> AGNDLLSCLTFNGVRNHTVFSADSDSDFNRFLHLSIQNPLFQNSLISKPSAIILPGSKEELSNTIRCIRKGSWTIRLRSGGASYEGLSYTSDTPFILIDLMNLNRVSIDLESETAWVESGSTLGELYYAITESSSKLGFTAGWCPTVGTGGHISGGGFGMMSRKYGLAADNVVDAILIDANGAILDRQAMGEDVFWAIRGGGGGVWGAIYAWKIKLLPVPEKVTVFRVTKNVAIDEATSLLHKWQFVAEELEEDFTLSVLGGADEKQVWLTMLGFHFGLKTVAKSTFDLLFPELGLVEEDYLEMS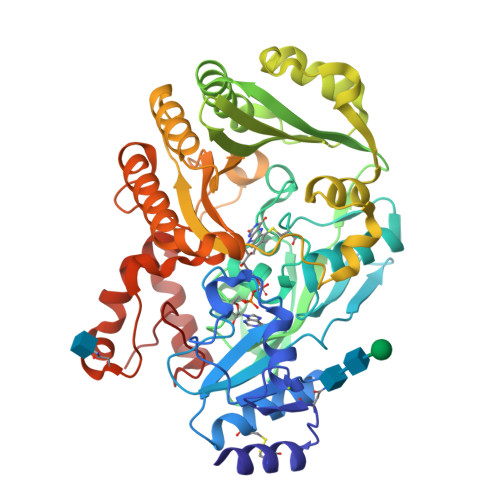WGESFAYLAGLETVSQLNNRFLKFDERAFKTKVDLTKEPLPSKAFYGLLERLSKEPNGFIALNGFGGQMSKISSDFTPFPHRSGTRLMVEYIVAWNQSEQKKKTEFLDWLEKVYEFMKPFVSKNPRLGYVNHIDLDLGGIDWGNKTVVNNAIEISRSWGESYFLSNYERLIRAKTLIDPNNVFNHPQSIPPMA>MQVSLPREDTVYIGGALWGPATTWNLYAPQSTWGTDQFMYLPAFQYDLGRDAWIPVIAERYEFVDDKTLRIYIRPEARWSDGVPITADDFVYALELTKELGIGPGGGWDTYIEYVKAVDTKVVEFKAKEENLNYFQFLSYSLGAQPMPKHVYERIRAQMNIKDWINDKPEEQVVSGPYKLYYYDPNIVVYQRVDDWWGKDIFGLPRPKYLAHVIYKDNPSASLAFERGDIDWNGLFIPSVWELWEKKGLPVGTWYKKEPYFIPDGVGFVYVNNTKPGLSDPAVRKAIAYAIPYNEMLKKAYFGYGSQAHPSMVIDLFEPYKQYIDYELAKKTFGTEDGRIPFDLDMANKILDEAGYKKGPDGVRVGPDGTKLGPYTISVPYGWTDWMMMCEMIAKNLRSIGIDVKTEFPDFSVWADRMTKGTFDLIISWSVGPSFDHPFNIYRFVLDKRLSKPVGEVTWA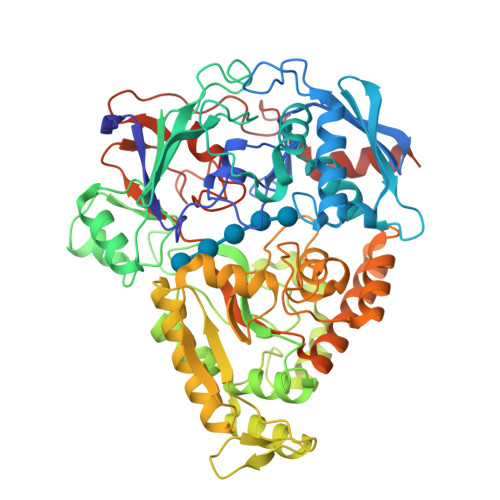GDWERYDNDEVVELLDKAVSTLDPEVRKQAYFRIQQIIYRDMPSIPAFYTAHWYEYSTKYWINWPSEDNPAWFRPSPWHADAWPTLFIISKKSDPQPVPSWLGTVDEGGIEIPTAKIFEDLQKATMHHHHHH[2x]> TRYKNAK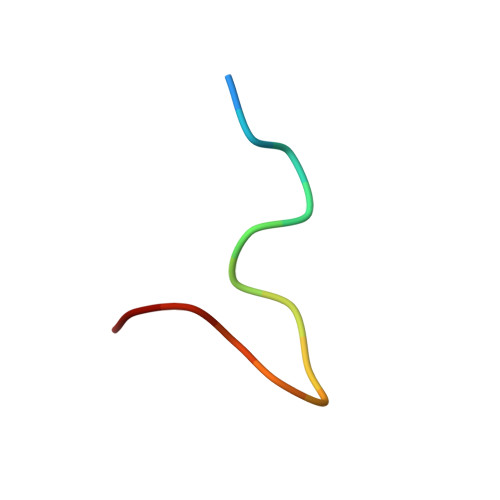MLPFAFGA> SITGISPITEYLASLSTYNDQSITFALEDESYEIYVEDLKKDEKKDKVLLSYYESQHPSNESGDGVDGKMLMVTLSPTKDFWLHANNKEHSVELHKCEKPLPDQAFFVLHNMHSNCVSFECKTDPGVFIGVKDNHLALIKVDSSENLCTENILFKLSET;> KFSKQSWGLENEALIVRCPRQGKPSYTVDWYYSQTNKSIPTQERNRVFASGQLLKFLPAAVADSGIYTCIVRSPTFNRTGYANVTIYKKQSDCNVPDYLMYSTVSGSEKNSKIYCPTIDLYNWTAPLEWFKNCQALQGSRYRAHKSFLVIDNVMTEDAGDYTCKFIHNENGANYSVTATRS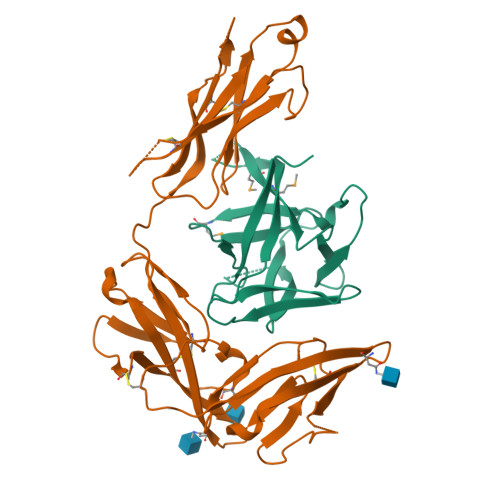FTVKDEQGFSLFPVIGAPAQNEIKEVEIGKNANLTCSACFGKGTQFLAAVLWQLNGTKITDFGEPRIQQEEGQNQSFSNGLACLDMVLRIADVKEEDLLLQYDCLALNLHGLRRHTVRLSRKHHHHHH>[2x]MENFPTEYFLNTTVRLLEYIRYRDSNYTREERIENLHYAYNKAAHHFAQPRQQQLLKVDPKRLQASLQTIVGMVVYSWAKVSKECMADLSIHYTYTLVLDDSKDDPYPTMVNYFDDLQAGREQAHPWWALVNEHFPNVLRHFGPFCSLNLIRSTLDFFEGCWIEQYNFGGFPGSHDYPQFLRRMNGLGHCVGASLWPKEQFNERSLFLEITSAIAQMENW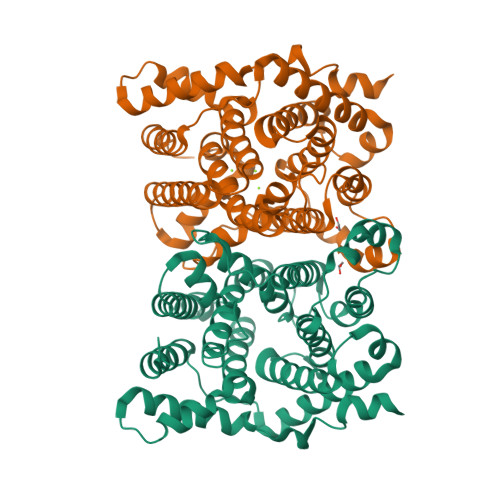MVWVNDLMSFYKEFDDERDQISLVKNYVVSDEISLHEALEKLTQDTLHSSKQMVAVFSDKDPQVMDTIECFMHGFVTWHLCDRRYRLSEIYEKVKEEKTEDAQKFCKFYEQAANVGAVSPSEWAYPPVAQLANVRSKDVKEVQKPFLSSIELVE>[2x]GSHMASFNGVSEAELLTKTLPDILTFNLDIVIIGINPGLMAAYKGHHYPGPGNHFWKCLFMSGLSEVQLNHMDDHTLPGKYGIGFT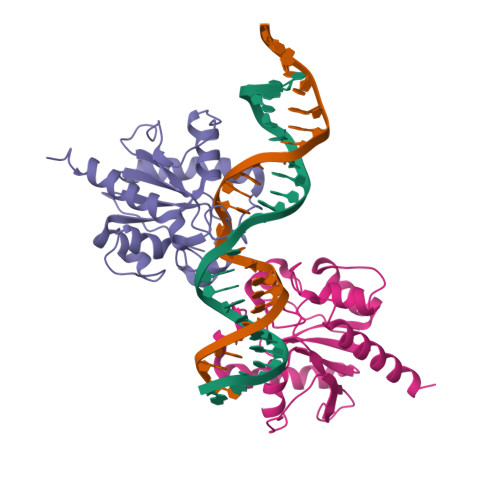NMVERTTPGSKDLSSKEFREGGRILVQKLQKYQPRIAVFNGKCIYEIFSKEVFGVKVKNLEFGLQPHKIPDTETLCYVMPSSSARCAQFPRAQDKVHYYIKLKDLRDQLKGIERNMDV> MSLSTMLVAEDLSAVGGISLSSALPVLTAMQYDVAALPTSLLSTHTSGYGTPAVVDLSTWLPQVFAHWTRAQLHFDQALIGYVGSVALCQQITTYLEQQTLSLLVVDPVLGDLGQLYQGFDQDYVAAMRQLIQQADVILPNTTEAALLTGAPYQVTPDLEVILPALQAQLKTGAHAVITDVQRADQIGCAWLDEAGHVQYCGARR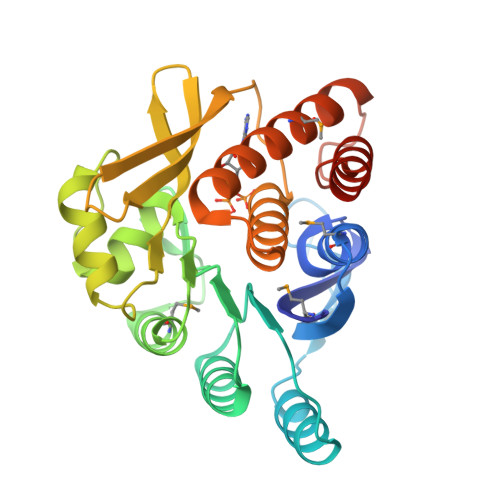LPGHYNGTGDTLAAVIAGLLGRGYPLAPTLARANQWLNMAVAETIAQNRTDDRQGVALGDLLQAILALNEGHHHHHH6-(2-aminopyrimidin-4-yl)-1H-indazol-3-amine | C11 H10 N6 | 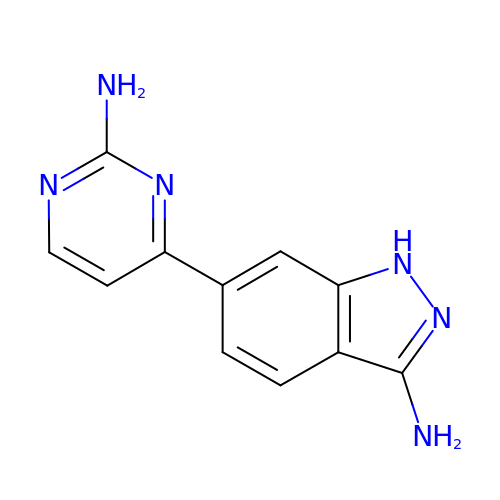QVWIVWPIJUYRRF-UHFFFAOYSA-N> GLIVDTRDVEERVHVMRKTKLAPTVAHGVFNPEFGPAALSNKDSRLNEGVVLDEV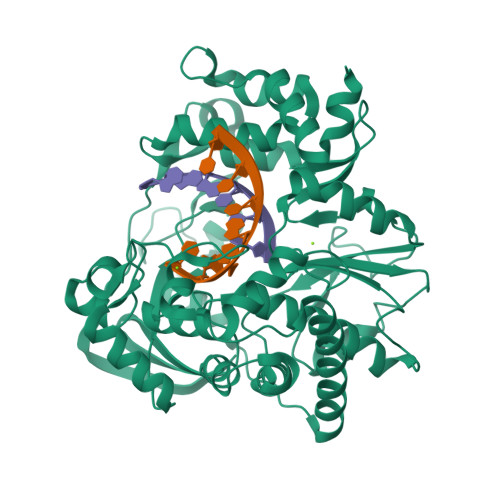IFSKHKGDTKMSAEDKALFRRCAADYASRLHSVLGTANAPLSIYEAIKGVDGLDAMEPDTAPGLPWALQGKRRGALIDFENGTVGPEVEAALKLMEKREYKFACQTFLKDEIRPMEKVRAGKTRIVDVLPVEHILYTRMMIGRFCAQMHSNNGPQIGSAVGCNPDVDWQRFGTHFAQYRNVWDVDYSAFDANHCSDAMNIMFEEVFRTEFGFHPNAEWILKTLVNTEHAYENKRITVEGGIPSGCSATSIINTILNNIYVLYALRRHYEGVELDTYTMISYGDDIVVASDYDLDFEALKPHFKSLGQTITPADKSDKGFVLGHSITDVTFLKRHFHMDYGTGFYKPVMASKTLEAILSFARRGTIQEKLISVAGLAVHSGPDEYRRLFEPFQGLFEIPSYRSLYLRWVNAVCGDAAALAH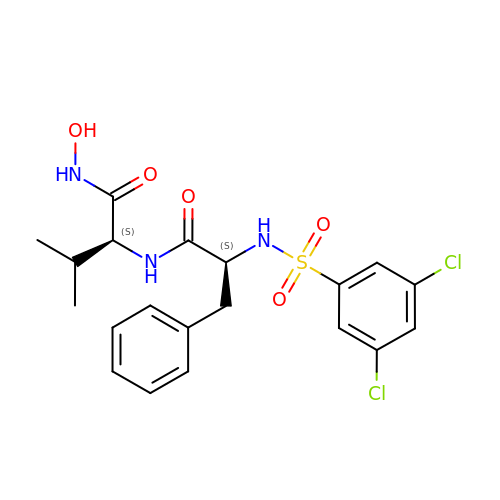N-[(3,5-dichlorophenyl)sulfonyl]-L-phenylalanyl-N-hydroxy-L-valinamide | C20 H23 Cl2 N3 O5 S | OEORWLJKQWVGLS-ROUUACIJSA-N2-amino-5-(5-aminopent-1-yn-1-yl)-7-{2-deoxy-5-O-[(S)-hydroxy{[(S)-hydroxy(phosphonooxy)phosphoryl]oxy}phosphoryl]-beta-D-erythro-pentofuranosyl}-3,7-dihydro-4H-pyrrolo[2,3-d]pyrimidin-4-one 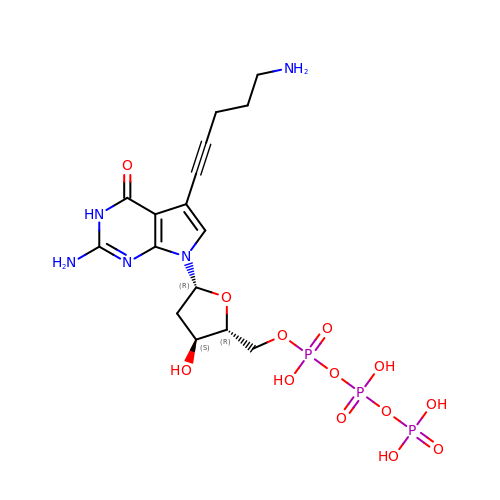| C16 H24 N5 O13 P3 | XIWGGMXHUSVMFH-QJPTWQEYSA-N> AKKETIDKVSDIVKEKLALGADVVVTADSEFSKLGADSLDTVEIVMNLEEEFGINVDEDKAQDISTIQQ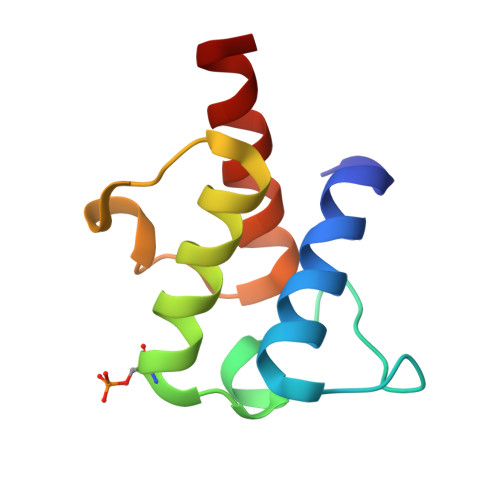AADVIEGLLEKKA>[2x]GMSPQSMLTSPQHP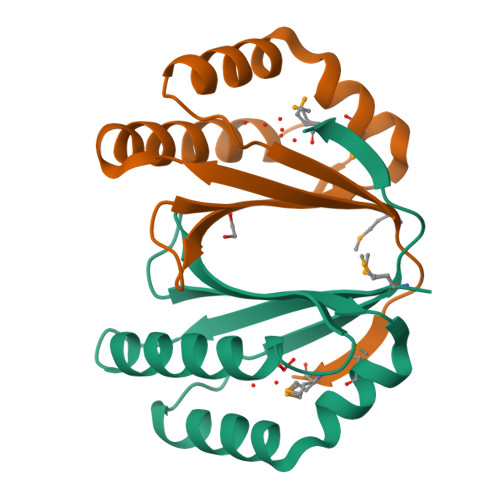RRTTMVISHGTLSASAEHAAHLRQLLVHIAQATRQEDGCLLYLVSEDLSQPGHFLITEHWDNLGAMHTHLALPGVTQAIDALKHLNVTDLKITAYEAGEAINIMG> MRQTLPCIYFWGGLLPFGMLCASSTTKCTVSHEVADCSHLKLTQVPDDLPTNITVLNLTHNQLRRLPAANFTRYSQLTSLDVGFNTISKLEPELCQKLPMLKVLNLQHNELSQLSDKTFAFCTNLTELHLMSNSIQKIKNNPFVKQKNLITLDLSHNGLSSTKLGTQVQLENLQELLLSNNKIQALKSEELDIFANSSLKKLELSSNQIKEFSPGCFHAIGRLFGLFLNNVQLGPSLTEKLCLELANTSIRNLSLSNSQLSTTSNTTFLGLKWTNLTMLDLSYNNLNVVGNDSFAWLPQLEYFFLEYNNIQHLFSHSLHGLFNVRYLNLKRSFTKQSISLASLPKIDDFSFQWLKCLEHLNMEDNDIPGIKSNMFTGLINLKYLSLSNSFTSLRTLTNETFVSLAHSPLHILNLTKNKISKIESDAFSWL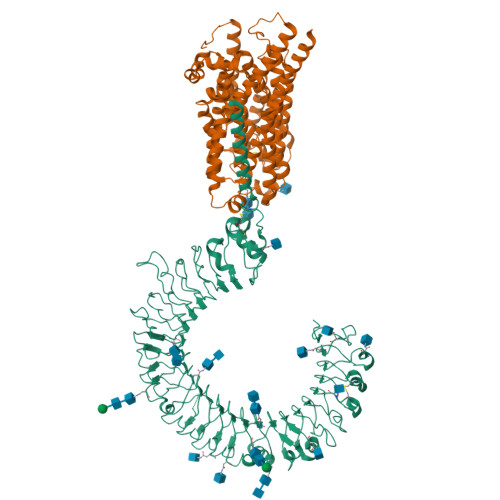GHLEVLDLGLNEIGQELTGQEWRGLENIFEIYLSYNKYLQLTRNSFALVPSLQRLMLRRVALKNVDSSPSPFQPLRNLTILDLSNNNIANINDDMLEGLEKLEILDLQHNNLARLWKHANPGGPIYFLKGLSHLHILNLESNGFDEIPVEVFKDLFELKIIDLGLNNLNTLPASVFNNQVSLKSLNLQKNLITSVEKKVFGPAFRNLTELDMRFNPFDCTCESIAWFVNWINETHTNIPELSSHYLCNTPPHYHGFPVRLFDTSSCKDSAPFELFFMINTSILLIFIFIVLLIHFEGWRISFYWNVSVHRVLGFKEIDRQTEQFEYAAYIIHAYKDKDWVWEHFSSMEKEDQSLKFCLEERDFEAGVFELEAIVNSIKRSRKIIFVITHHLLKDPLCKRFKVHHAVQQAIEQNLDSIILVFLEEIPDYKLNHALCLRRGMFKSHCILNWPVQKERIGAFRHKLQVALGSKNSVH;> MEAEPPLYPMAGAAGPQGDEDLLGVPDGPEAPLDELVGAYPNYNEEEEERRYYRRKRLGVLKNVLAASAGGMLTYGVYLGLLQMQLILHYDETYREVKYGNMGLPDIDSKMLMGINVTPIAALLYTPVLIRFFGTKWMMFLAVGIYALFVSTNYWERYYTLVPSAVALGMAIVPLWASMGNYITRMAQKYHEYSHYKEQDGQGMKQRPPRGSHAPYLLVFQAIFYSFFHLSFACAQLPMIYFLNHYLYDLNHTLYNVQSCGTNSHGILSGFNKTVLRTLPRSGNLIVVESVLMAVAFLAMLLVLGLCGAAYRPTEEIDLRSVGWGNIFQLPFKHVRDYRLRHLVPFFIYSGFEVLFACTGIALGYGVCSVGLERLAYLLVAYSLGASAASLLGLLGLWLPRPVPLVAGAGVHLLLTFILFFWAPVPRVLQHSWILYVAAALWGVGSALNKTGLSTLLGILYEDKERQDFIFTIYHWWQAVAIFTVYLGSSLHMKAKLAVLLVTLVAAAVSYLRMEQKLRRGVAPRQPRIPRPQHKVRGYRYLEEDNSDESDAEGEHGDGAEEEAPPAGPRPGPEPAGLGRRPCPYEQAQGGDGPEEQ> GGGCUGCACUUCGGUGCUGCC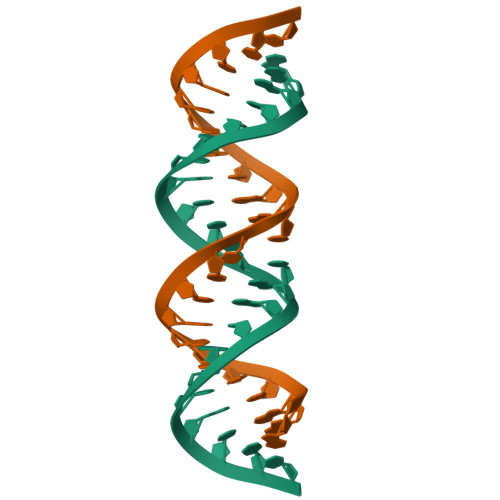C> MLTEGISIQSYDGHTFGALVGSPAKAPAPVIVIAQDIFGVNAFMRETVSWLVDQGYAAVCPDLYARQAPGTALDPQDERQREQAYKLWQAFDMEAGVGDLEAAIHYARHQPYSNGKVGLVGYSLGGALAFLVAAKGYVDRAVGYYGVGLEKQLNKVPEVKHPALFHMGGQDHFVPAPSRQLITEGFGANPLLQVHWYEEAGHSFARTSSSDYVASAAALANERTLDFLAPLQ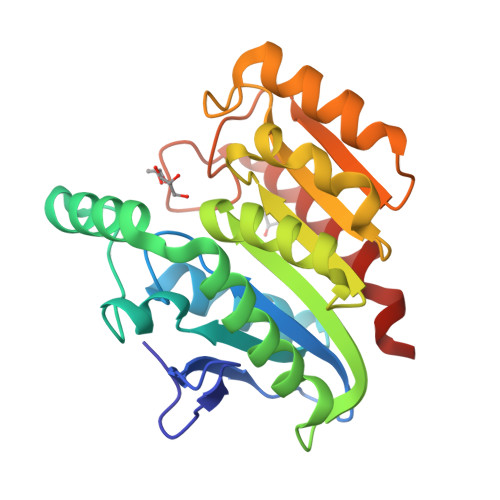SNKP>MAHHHHHHVDDDDKMVTDQRWLIDKSALVRLTDSPDMEIWSNRIERGLVHITGVTRLEVGFSAECGEIARREFREPPLSAMPVEYLTPRIEDRALEVQTLLADRGHHRGPSIPDLLIAATAELSGLTVL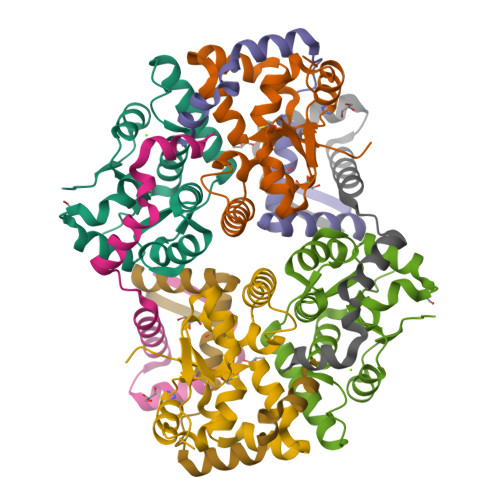HVDKDFDAIAALTGQKTERLTHRPPSA[2x];>[2x]MSDVLIRDIPDDVLASLDAIAARLGLSRTEYIRRRLAQDAQTARVTVTAADLRRLRGAVAGLGDPELMRQAWR>MTEETISQAVPPVRDWPAVDLPGSDFDPVLTELMREGPVTRISLPNGEGWAWLVTRHDDVRLVTNDPRFGREAVMDRQVTRLAPHFKPARGAVGFLDPPDHTRLRRSVAAAFTARGVERVRERSRGMLDELVDAMLRAGPPADLTEAVLSPFPIAVICELMGVPATDRHSMHTWTQLILSSSHGAEVSERAKNEMNAYFSDLIGLRSDSAGEDVTSLLGAAVGRDEITLSEAVGLAVLLQIGGEAVTNNSGQMFHLLLSRPELAERLRSEPEIRPRAIDELLRWIPHRNAVGLSRIALEDVEIKGVRIRAGDAVYVSYLAANRDPEVFPDPDRIDFERSPNPHVSFGFGPHYCPGGMLARLESELLVDAVLDRVPGLKLAVAPEDV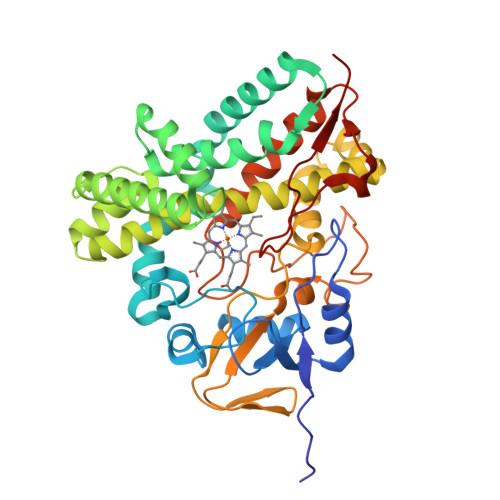PFKKGALIRGPEALPVTWHHHHHH[2x]>[4x]MKCTIPEQQKVILIDEIGGYDVIKYEDYPVPSISEEELLIKNKYTGVNYIESYFRKGIYPCEKPYVLGREASGTVVAKGKGVTNFEVGDQVAYISNSTFAQYSKISSQGPVMKLPKGTSDEELKLYAAGLLQVLTALSFTNEAYHVKKGDYVLLFAAAGGVG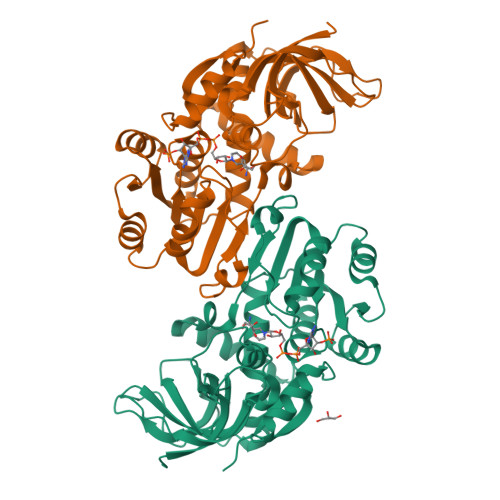LILNQLLKMKGAHTIAVASTDEKLKIAKEYGAEYLINASKEDILRQVLKFTNGKGVDASFDSVGKDTFEISLAALKRKGVFVSFGNASGLIPPFSITRLSPKNITLVRPQLYGYIADPEEWKYYSDEFFGLVNSKKLNIKIYKTYPLRDYRTAAADIESRKTVGKLVLEIPQ> MSGFLLRLAGPMQSWGEHSMFGERDTLPYPSRSGLIGMFAAAQGVRRGDPLDRYKELKFTVRVDRPGVRLVDFHTIGGGLPKERTVPTAAGERRDPKKATIVTSRSYLADAVFTVAVTGPEADTIADALAAPYWQPYLGRRAFVPDPLLVLRRRVADPVRELVEAVPLPHRRVEEDAATVLVDLIYEEGEYPDTRTLTVLNDVPLSFDSKSRRYSTRQIRVVPT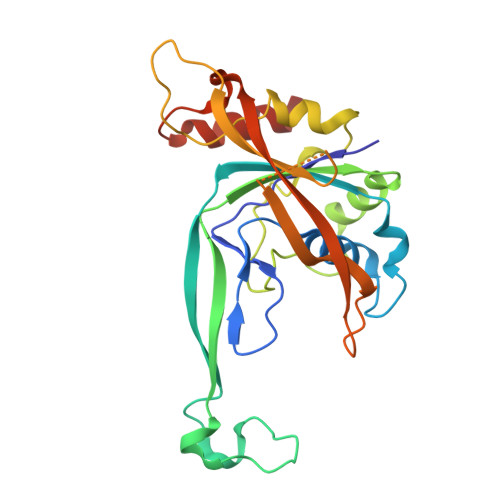EVPATLVAGPGRDYQNKLFTYVKQCAEEAA>KEAETQQKLANVVILATGGTIAGAGASAANSATYQAAKLGVDKLIAGVPELADIANVRGEQVMQIASESISNDDLLKLGKRVAELAESKDVDGIVITHGTDTLEETAFFLNLVEKTDKPIVVVGSMRPGTAMSADGMLNLYNAVAVASDKQSRGKGVLVTMNDEIQSGRDVSMAVNIKTEAFKSAWGPMGMVVEGKSYWFRLPAKRHTVNSEFDIKQISSLPQVDIAYGYGNVTDTAYKALAQNGAKALIHAGTGNGSVSSRVVPALQEL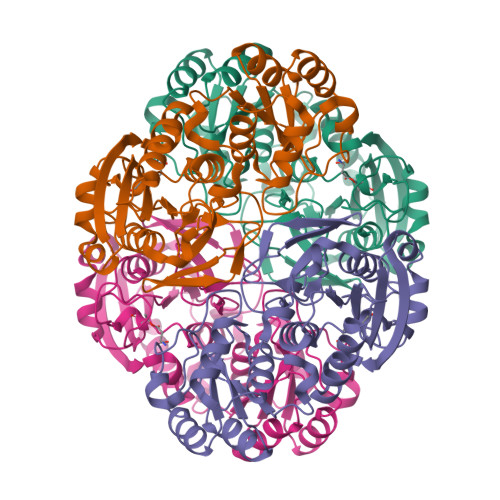RKNGVQIIRSSHVNQGGFVLRNAEQPDDKNDWVVAHDLNPQKARILAMVAMTKTQDSKELQRIFWEY[4x]> MEDDMACVKDLVSKYLADNERLSRQKLAFLVQTEPRMLLMEGLKLLSLCIEIDSCNANGCEHNSEDKSVERILHDHGILTPSLCFVVPDGYKLTGNVLILLECFVRSSPANFEQKYIEDFKKLEQLKEDLKSVDINLIPLIDGRTSFYNEQIPDWVNDKLRDTLFSLLRYAQESNSLFEESEYSRLCESLSMTSGRLSGVESLNVLLDNRSSHYEEIIASCHQGINNKLTAHEVKLQIEEEYQVFRNRLRKGEITGQFLKVDKSRLLNDFNNLYVDEVTATKDNIEHLIYQFKRASPILRFLYANIGEGNGEERHHTIKECQMQYWRSFLNKVKSLRILNTRRKLLLIFDALILLASIHDQTRHKCSKGWLGSCFISVNDRLVSLESTKRDLEKWVGRRQQSERSNTIQPPDKNQILISMFQKTILKATAALKDVGISVEHYKINMEVICPDSYDLILNFDVSGVVPTISYQRTEDEKFPFIMGGVELLESTDLERLSSLSLALVNSMKTSSTVKLRQNEFGPARYQVVRCKEAYCQEFLLSGAEFQLIYQKTGECSKCYAINDNRVGEICSFYADPKRYFPAIFSAEVLQTTVSTMISWVKDCSELEEQLCNINSLTKMILVLILAHPSKRSQKLLQNLRYFIMAYVSDYHHKDLIDKLREELITDVEFLLYRLVRALVNLILSEDVKSMMTNRFKFILNISYMCHFITKETPDRLTDQIKCFEKFLEPKLEFGHVSINPADVATEEELDDMVYNAKKFLSKEGCTSIKGPDYKKPGVSKRFLSLLTSSFNNGSLFKESEVKREIKDPLVTSGCATALDLASNKSVVVNKYTDGSRVLNYDFNKLTALAVSQLTEVFSRKGKHLLNKQDYDYKVQQAMSNLVLGPRQNKVGADEADLDEILLDGGASVYFDQLKETVERIIDQYREPVKPGSNPNGGDQPSVNDLDEVVPNKFYIRLIKGELSNHMVEDFDYDVLPGNFYEEFCDAVYKNNKLKERYFYCGQMSQCPIGELTKAVATRTYFDQEYFQCFKSILLIMNANTLMGRYTHYKSRNLNFKFDMGRLSDDVRISERESNSEALSKALSLTNCTTAMLKNLCFYSQESPQSYSSTGPDTGRLKFSLSYKEQVGGNRELYIGDLRTKMFTRLIEDYFEALSLQLSGSCLNNEREFENAILSMKLNVSLAHVSYSMDHSKWGPMMCPFLFLATLQNLIFLSKDLQADIKGRDYLSTLLTWHMHKMVEIPFNVVSAMMKSFIKAQLGLKKKTTQSITEDFFYSNFQIGVVPSHVSSILDMGQGILHNTSDFYALISERFINYAISCICGGTIDAYTSSDDQISLFDQVLTELMQRDPEEFKTLIEFHYYMSDQLNKFVSPKSVIGRFVAEFKSRFYVWGDEVPLLTKFVAAALHNIKCKEPHQLAETIDTIIDQSVANGVPVHLCNLIQKRTLSLLQYARYPIDPFLLNCETDVRDWVDGNRSYRIMRQIERLIPDACGRIRSMLRKLYNKLKTGQLHEEFTTNYLSSEHLSSLSNLCELLGVEPPSESDLEFSWLNLAAHHPLRMVLRQKIIYSGAVNLDDEKVPTIVKTIQNKLSSTFTRGAQKLLSEAINKSAFQSSIASGFVGLCRTLGSKCVRGPNKESLYIKSIQS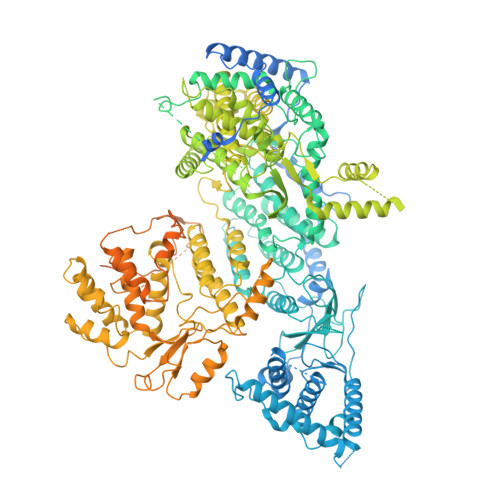LISDIQGIEPLIDSHGVQYWRVPLNIRDGNEGVISYFRPLLWDYMCISLSTAIELGAWVLGEPKKVRVLEFFKHNPCDYFPLKPAASKLLEDRVGLNHIIHSLRRLYPSVFEKHILPFMSDLASTKMKWSPRIKFLDLCVALDVNCEALSLVSHIVKWKREEHYIVLSSELRLSHTRTHEPMVEERVVSTSDAVDNFMRQIYFESYVRSFVATTRTLGSFTWFPHKTSVPEGEGLQRLGPFSSFVEKAIHKGIERPMFKHDLMMGYAWIDFDIEPARFNHNQLIASGLVGPRFDSLEDFFDAVESLPPGSAKLSQTVRFRIKSQDASFKESFAIHLDYTGSINQQTKYLVHEVSAMYSGAVSPCVLSDCWRLVLSGPTFKGKSAWYVDTEIVNEFLTDTNQLGHVTPVEIVVDMEKLQFTEYDFVLVGPCVEPVPLVVHRGGLWECDKKLASFTPVVQDQDLEMFVKEVGDSSLDLLIGALSAMILDRLKLRMQWSEVDIVSMLKAAMPSNSVKVLNAVLEAVDDWVDFKGYALCYSKSRKKVMVHSSGGKLRLKGRTCEELVKEDEGIEDIE>DAHSLRCNLTIKDPTPADPLWYEAKCFVGEILILHLSNINKTMTSGDPGETANATEVKKCLTQPLKNLCQKLRNKVSNTKVDTHKTNGYPHLQVTMIYPQSQGRTPSATWEFNISDSYFFTFYTENMSWRSANDESGVIMNKWKD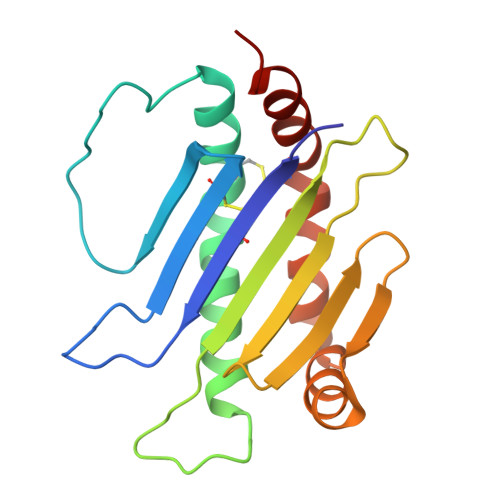DGEFVKQLKFLIHECSQKMDEFLKQSKEK[5x]>[2x]TSDPALQYERITPEWTAEAVIEGCAPLTPLNMTRSIAEMHMEHPPLGITRFFKELGYKIAKKKGSEGTRRNRFVGQLIEPLRRVLERHHLFGAWQLTSTTPRAVFNIFRSKVDRAPVELHSHYPGLKKMYDILADLWLERYGSMKRLTEDEMASAINRRGAMGYQMDNRNYGDLGAYWDSGDWRQDVNTFKRALLSGTPTHAVYNTTAKKEKTKNLTRQVNKGSRIIQYLPADARLYELKVLGGLHKYLEKCGWSVAGQGLYKYGDRVKKSMDATGAAISEDVAGWDTKISKGLLTLESHMFTKLAEDEEMAREIHHLYRLYADPHMVVQREIEGEVHDVLLRGRGQVSSGRQPTYAANTITNFITTTYGMAMTLGIPEADWPRLIRNLTDERGNRRLLVSGDDKVLFLRGDEARVYASSAYRTSNDMGLVRKDMALEQESEIIVDVKEISFCSHRYWPVKYGNEIHYMPVRDVGEIFAKATMALG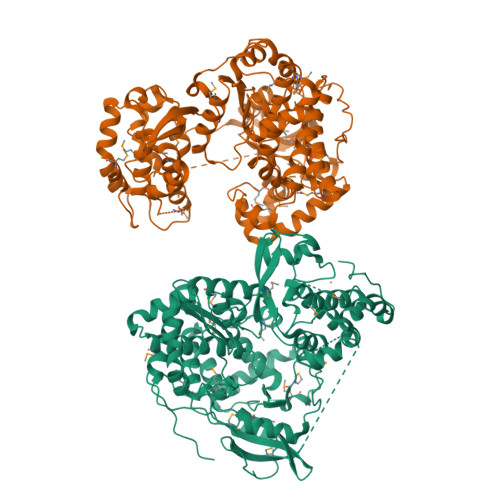VYKDDMTQEAWARVQGLNMLVNYHHIPECRMLALAILSVTRIGLNLKGVTKGWMMSTEWLRDDLAPDTIHALITEGRTSGWDQLGYVDFKDRKGILLRPDTSYKNWRRDLPGKVRQLREDGQYKDWLQRMAVFG> GSHMLKGQEFAPSHQQVYAPLRADGDKPRAHLTVVRQTPTQHFKNQFPALHWEH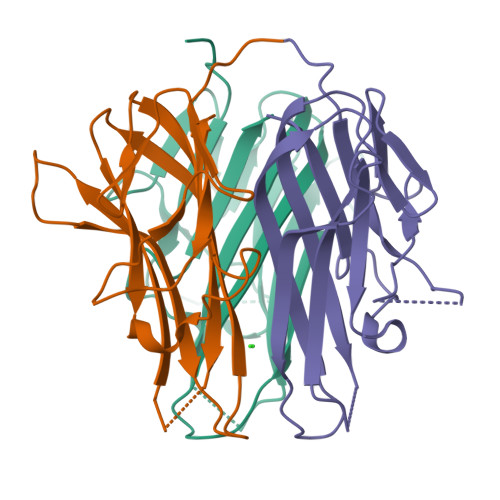ELGLAFTKNRMNYTNKFLLIPESGDYFIYSQVTFRGMTSECSEIRQAGRPNKPDSITVVITKVTDSYPEPTQLLMGTKSVCEVGSNWFQPIYLGAMFSLQEGDKLMVNVSDISLVDYTKEDKTFFGAFLL> MVIVPEGTQLDEKQHIV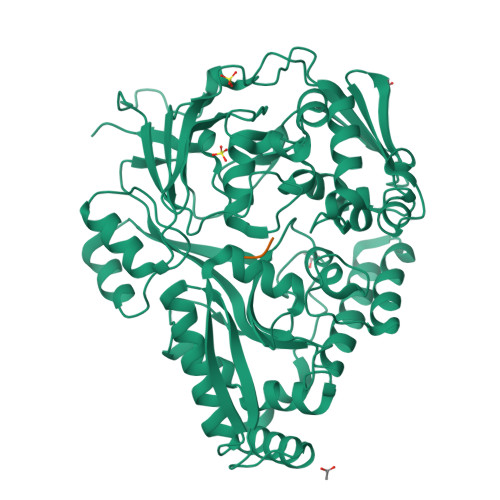INNGAEPQSFDPHKTEGVPESNVAYQLLEGLVTSDSEGKLQPGAAESWENTPDFKTWTFHLRKDAKWSNGDPVTAHDFVFAWRRLVDPATAAPYASYLSYLQVENAQDIIDGKKKPAELGVEAKDDYTFVVHATNPVPYAVSLTTHQSLLPLPQKVVEKLGDAWVKKENYVGNGAYKLANHIINEKIEFERNPLYWNDKETVINSATFLAIENPSTDVARYRAGDLDMTSYGLPPEQFAKLKKELLGEVYVTRTLGTYSYELNNKKAPFDNVNIRKALNLSLDRNVITDKVLGQGQTPTYVFTPTYIEEGHLIQQPAYSKEPMAQRNEEAIKLLEEAGYSKANPLKFSILYNTNENHKKVAIAAASMWKANTKGLIDVKLENQEWKTYIDSRRAGRYDVARAGWHADYNQATTFGNYFLSNSSNNTAKYANPEYDKAMAESYAATDAEGRAKAYAKAEEILGKDYGIVPIFNYVNPRLVKPYVKGYSGKDPQDHIYLRNLYIIKHLEHHHHHH;> LGG>[6x]EPEPQMVLSPLTSAAIFLVVTIDSGGEDTVRDLLSDVASLERAVGFRAQPDGRLSCVTGIGSEAWDRLFSGARPAGLHPFRELDGPVHRAVATPGDLLFHIRASRLDLCFALAT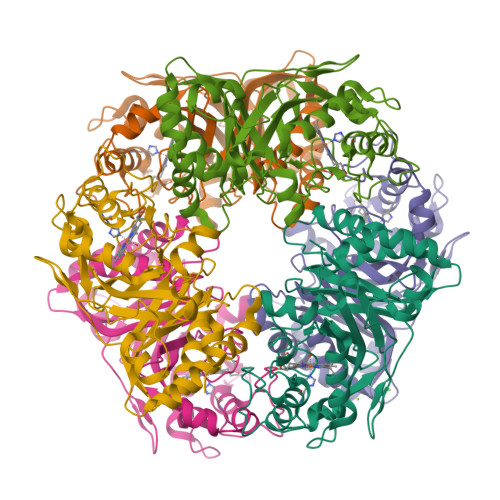EIMGRLRGAVTPQDEVHGFKYFDERDMLGFVDGTENPTGAAARRAVLVGAEDPAFAGGSYAVVQKYLHDIDAWEGLSVEAQERVIGRRKMTDVELSDDVKPADSHVALTSVTGPDGSDLEILADNMPFGSVGREEFGTYFIGYARTPEVTETMLERMFLGTASAPHDRILDFSTAVTGSLFFTPAADFLEDLS> GSHMKEVSEHCSHMIGNGHLKVLQQLIDSQMETSCQIAFEFVDQEQLDDPVCYLKKAFFLVQDIIDETMRFKDNTPNANATERLQELSNNLNSCFTKDYEEQNKACVRT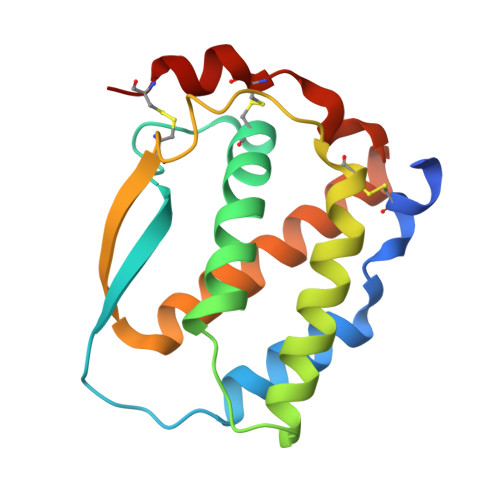FHETPLQLLEKIKNFFNETKNLLEKDWNIFTKNCNNSFAKCSSR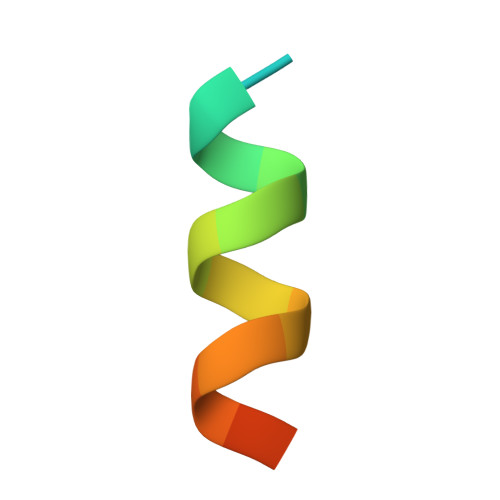> TNMGLEAIIRKALMGKY>MTTELNQGEQFVADFRANAAALTTANAYNPEDEHDACGVGFIAAIDGKPRRSVVEKGIEALKAVWHRGAVDADGKTGDGAGIHVAVPQKFFKDHVKVIGHRAPDNKLAVGQVFLPRISLDAQEACRCIVETEILAFGYYIYGWRQVPINVDIIGEKANATRPEIEQIIVGNNKGVSDEQFELDLYIIRRRIEKAVKGEQINDFYICSLSARSIIYKGMFLAEQLTTFYPDLLDERFESDFAIYHQRYSTNTFPTWPLAQPFRMLAHNGEINTVKGNVNWMKAHETRMEHPAFGTHMQDLKPVIGVGLSDSGSLDTVFEVMVRAGRTAPMVKMMLVPQALTSSQTTPDNHKALIQYCNSVMEPWDGPAALAMTDGRWVVGGMDRNGLRPMRYTITTDGLIIGGSETGMVKIDETQVIEKGRLGPGEMIAVDLQSGKLYRDRELKDHLATLKPWDKWVQNTTHLDELVKTASLKGEPSDMDKAELRRRQQAFGLTMEDMELILHPMVEDGKEAIGSMGDDSPIAVLSDKYRGLHHFFRQNFSQVTNPPIDSLRERRVMSLKTRLGNLGNILDEDETQTRLLQLESPVLTTAEFRAMRDYMGDTAAEIDATFPVDGGPEALRDALRRIRQETEDAVRGGATHVILTDEAMGPARAAIPAILATGAVHTHLIRSNLRTFTSLNVRTAEGLDTHYFAVLIGVGATTVNAYLAQEAIAERHRRGLFGSMPLEKGMANYKKAIDDGLLKIMSKMGISVISSYRGGGNFEAIGLSRALVAEHFPAMVSRISGIGLNGIQKKVLEQHATAYNEEVVALPVGGFYRFRKSGDRHGWEGGVIHTLQQAVTNDSYTTFKKYSEQVNKRPPMQLRDLLELRSTKAPVPVDEVESITAIRKRFITPGMSMGALSPEAHGTLNVAMNRIGAKSDSGEGGEDPARFRPDKNGDNWNSAIKQVASGRFGVTAEYLNQCRELEIKVAQGAKPGEGGQLPGFKVTEMIARLRHSTPGVMLISPPPHHDIYSIEDLAQLIYDLKQINPDAKVTVKLVSRSGIGTIAAGVAKANADIILISGNSGGTGASPQTSIKFAGLPWEMGLSEVHQVLTLNRLRHRVRLRTDGGLKTGRDIVIAAMLGAEEFGIGTASLIAMGCIMVRQCHSNTCPVGVCVQDDKLRQKFVGTPEKVVNLFTFLAEEVREILAGLGFRSLNEVIGRTDLLHQVSRGAEHLDDLDLNPRLAQVDPGENARYCTLQGRNEVPDTLDARIVADARPLFEEGEKMQLAYNARNTQRAIGTRLSSMVTRKFGMFGLQPGHITIRLRGTAGQSLGAFAVQGIKLEVMGDANDYVGKGLSGGTIVVRPTTSSPLETNKNTIIGNTVLYGATAGKLFAAGQAGERFAVRNSGATVVVEGCGSNGCEYMTGGTAVILGRVGDNFAAGMTGGMAYVYDLDDSLPLYINDESVIFQRIEVGHYESQLKHLIEEHVTETQSRFAAEILNDWAREVTKFWQVVPKEMLNRLEVPVHLPKAISAE[4x];>[4x]MANQRMLGFVHTAQRMPDKRPAAERRQDFAEIYARFSDERANEQANRCSQCGVPFCQVHCPVSNNIPDWLKLTSEGRLEEAYEVSQATNNFPEICGRICPQDRLCEGNCVIEQSTHGAVTIGSVEKYINDTAWDQGWVKPRTPSRELGLSVGVIGAGPAGLAAAEELRAKGYEVHVYDRYDRMGGLLVYGIPGFKLEKSVVERRVKLLADAGVIYHPNFEVGRDASLPELRRKHVAVLVATGVYKARDIKAPGSGLGNIVAALDYLTTSNKVSLGD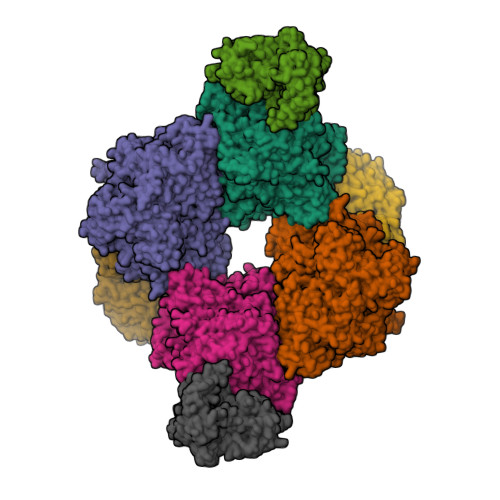TVEAYENGSLNAAGKHVVVLGGGDTAMDCVRTAIRQGATSVKCLYRRDRKNMPGSQREVAHAEEEGVEFIWQAAPEGFTGDTVVTGVRAVRIHLGVADATGRQTPQVIEGSEFTVQADLVIKALGFEPEDLPNAFDEPELKVTRWGTLLVDHRTKMTNMDGVFAAGDIVRGASLVVWAIRDGRDAAEGIHAYAKAKAEAPVAVAAE> GEHIPGTLRFRLSPAARNILEKHSLDASQGTATGPRGIFTKEDALKLVQLKQTGKILEHH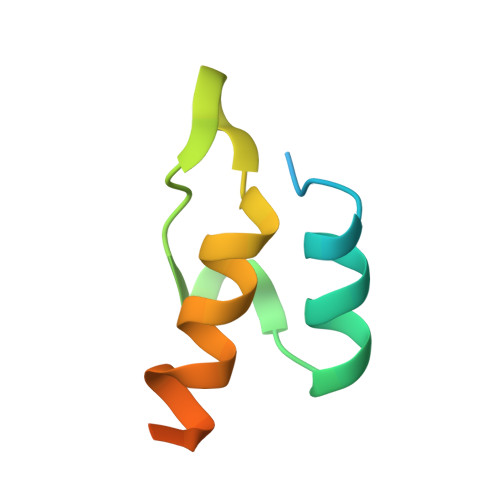HHHH>[10x]DYKDDDDKLDRADILYNIR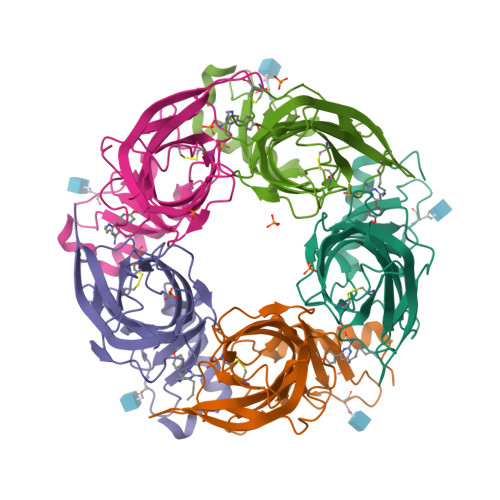QTSRPDVIPTQRDRPVAVSVSLKFINILEVNEITNEVDVVFWQQTTWSDRTLAWNSSHSPDQVSVPISSLWVPDLAAYNAISKPEVLTPQLARVVSDGEVLYMPSIRQRFSCDVSGVDTESGATCRIKIGSWTHHSREISVDPTTENSDDSEYFSQYSRFEILDVTQKKNSVTYSCCPEAYEDVEVSLNFRKKGRSEI Some animals such as molluscs and arthropods have blue blood because they utilize hemocyanin, a type-3 copper-containing protein that freely dissolves in hemolymph for oxygen transportation. Molluscan hemocyanins form decamers or multidecamers of 330–550 kDa subunits, which associate into huge cylindrical supermolecules with molecular masses varying from 3.5 to 13.5 MDa. Subunits of most molluscan hemocyanins consist of an N-terminal segment of six paralogous functional units (FUs; a-b-c-d-e-f) and a C-terminal segment with a varying number of FUs. Ten copies of the N-terminal segment (FUs a, b, c, d, e and f) thereby form a conserved cylinder wall, whereas the C-terminal segments form several inner-collar domains, located on the inner periphery of the cylinder.

Type 4 molluscan hemocyanin (squid type) is exceptional since this is the only molluscan hemocyanin type with an additional FU (FU-d*) within the N-terminal segment that usually forms the cylinder wall. Therefore, we constructed the entire structure model by rigid-body fitting. Our structure revealed a striking asymmetric inner-collar architecture and a conserved symmetric cylinder wall. 5 symmetry that is shifted towards one cylinder opening (northern hemisphere of the lumen). In TpH, the FU-gs form typical FU dimers, but in this case the dimers unusually occupy the northern and southern hemispheres of the inner space alternately [cyan FUs in Figs. 1(e) and 2(b)]. FU-d*s do not form dimers, instead single copies fill void spaces between the FU-g dimers. The segment of the wall FUs (a-b-c-d,e-f) is invariant for all ten protomers and there are two different possible conformations for each FU-g and FU-d* within a single protomer, thereby resulting in four different protomer types, namely conformers 1, 2, 3 and 4.

>[10x]NLLRKNVDTLTPDEILNLQVSLRAMQDDEGASGYQAISAYHGEPADCKAADGSTIVCCLHGMPTFPMWHRLYLVQFEQALVAHGSTLGIPYWDWTKPMTQLPELVQHPLFIDPTGKKAKKNVFYSGEIKFENKVTARAVDARLYQASQEGQKNFLLEGVLNALEQEDFCHFEVQLEVAHNPIHYLVGGRFTHSMSSLEYTSYDPLFFLHHSNVERHFALWQALQKHRGLPTRPNCGLNLFHSPMEPFGRDTNPFAITKDNSKASSLFDYEHLGYAFDDLSLNGMTIEELEALLKQRRSGARAFANFRLGGIKTSANVRIKLCIPTEDKRQSDNCDNDAGQFFILGGTNEMPWNFAFPYLHEITDTVLSLGLALDSNYYVTAEVTAINGTLMPTQTIPRPIVTYIPPQGFKDVNMVNMDTSSLRFRKDISSLTTEEEYELRVAMERFMSDKSINGYQALAEFHGLPAKCPRPDALNRVACCIHGMATFPHWHRLVVMQFENALFTRGSPIGVPYWDWTKPFTALPSLLADETYVDPYTKETKPNPFFKAPIEFLKAGVHTSRQIDERLFKQPSKGDHGFLYDGLSLAFEQDDFCDFEVQFEVTHNSIHAWTGGSEPYSMSSLHYTSFDPMFWLHHSQVDRLWAIWQALQIQRGKPYKTYCANSEVYRPMKPFAFKSPLNNDEKTREHSVPTDVYDYQAELAYTYDTLFFGGLSIRELQRYVEEAKSKDRVFAGFLLMGIQTSANVDLFVVAGGNEFFVGSIAVLGGSKEMTWRFDRVYKHEITDALGALGVDMFAEYTLRVDIKDVNGTALPPTAIPPPIVIFVPGIADANVKFDEQHRSRKNVDSMTVSEMNALRTAMAAFAADKEVTGYQQVAAFHGSTQWCPSPDAAQKYACCHHGMATFPHWHRLIALNFENGLRRNGWSGGLPYWDWTRPIDALPALVLEAEYTDANGEAKPNPFFSGAIDSIGASTSRAPTEALYEKPDFGKYTHLANEIISALEQEDFCDFEVQYEIAHNHIHALVGGTEAVSMASLEYSAFDPIFMLHHSNVDRIWATWQALQKFRGKAYNSANCAIEILRKPMSPFSLASDINPDAMTREYSVPFDVFNYKKNFHYEYDTLELNGLSIXQLSREINRRKAKNRVXVTFMLEGLKKSLLVEYFIAADGTDQKMKAGEFYVLGSENEMPWKFDRPYKSDITYVMDAMKLHYTDKYHVELRITDMTGAEVTDLKLVTSVIYEPGIGNFGEGRRWISPITSASRIRKNLLDFEDGEMESLRNAFKQMADEGRYEEIASFHGVPAQCPSEDGTMVHTCCLHGMPVFPHWHRLYVSLVEDELLARGSGVAVPYWDWVEPFDELPRLINEATFYNSRTLQIEPNPFFKGKISFENAETDRDTQPELFGNRYLYDHTLFVFEQTDFCEFEVHYEVLHNTIHSWLGGRDVHSMSSLDYAAYDPVFFLHHSNVDRLWAIWQELQRYRKLSYNEANCALPLMNQPMRPFSNSTANNDRLTFTNSRPNDVFDYQNVLHYKYDTLNFAGLSIPQLERILQKNQGRDRIFAGFLLHGIKASADVRIYICVPTGIGEENCGNYAGIFSVLGGETEMPWQFDRLFRYEITDELKKLGLNQNSHFRVEMELTAVNGSKITQKIFPNPTIIFVPSDVEFEEDTWRDVVTSANRIRRNLKDLSKEDMFSLRAAFKRMTDDGRYEEIAAFHGLPAQCPNADGSNIHTCCLHGMPTFPHWHRLYLSLVENELLARGSDVAVPYWDWIEPFDSLPGLISDETYKHPKTNEDIENPFHHGKISFADAVTVRKPRDQLFNNRYLYEHALFAFEHTDFCDFEVHFEVLHNSIHSWIGGPNPHSMSSLDFAAYDPIFFLHHSTVDRLWAIWQDLQRYRKLDYNVANCALNLLNDPMRPFNNKTANQDHLTFTNSRPNDVFDYQNSLNYKFDSLSFSGLSIPRLDDLLESRQSHDRVFAGFWLSGIKASADVNIHICVPIGVEHEDCDNYAGTFAVLGGETEMPWAFDRLFRYEISDEMKKLQLTEDSKFRLTTNIIASNGSKVSNDIFPTPTVIFVPKKERTEQVSTTKSVRGNLVRKNVDRLSLQEINSLIHALKRMQKDRSSDGFETIASFHALPPLCPNPTAKHRHACCLHGMATFPQWHRLYVVQFEHSLNRHGAIVGVPYWDWTYPMTEVPGLLTSEKYTDPFTGIETFNPFNHGHISFISPETMTTREVSEHLFEQPALGKQTWLFNNIILALEQTDYCDFEVQFEIVHNSIHSWLGGKELYSLNHLHYAAYDPAFFLHHSNVDRLWVVWQELQKFRGLPAYESNCAIELMSQPLKPFSFGAPYNLNPVTTKYSKPSDVFNYKQNFHYEYDMLEMNGMSIAQLESYIRQERQKDRVFAGFLLEGFGSSAYATFQVCPDVGDCYEGSHFSVLGGSTEMPWAFDRLYKMEITDILQAMDLKFDSHFTIKTKIVAHNGTELPESLLPEATIVRIPPSAQNLEVAIPLNRIRRNINSLESRDVQNLMSALKRLKEDESDFGFQTIAGYHGSLMCPTPEAPEYACCLHGMPTFMHWHRVYLLHFEESMRRHGASVAVPYWDWTMPSDNLPSLLGDADYYDAWTDSVIENPFLRGHIKYEDTYTVREIQPELFALAEGQKESTLFKDVMLMFEQEDYCDFEVQAEVIHNSIHYLIGGHQKYAMSSLMFSSFDPIFYVHHSMVDRLWAIWQELQKHRKLPHDKAYCALDQMAFPMKPFIWESNPNPTTRAVSTPSKLFDYKSLGYDYDHLNFHGMSIGQLEALIQKQKKADRVFAGFLLHGIKISADVHLKICIEADCQEAGVIFVLGGETEMPWHFDRNYKMDITDVLKKRNIPPEALFEHDSKIRLEVEIKSVDGAVLDPNSLPKPSLIYAPAKGLIIQQVGEYDAGSMVRKNVNSLTPSEIENLRNALAAVQADKTDAGYQKIASFHGMPLSCQYPDGTAFACCQHGMVTFPHWHRLYMKQMEDALKAKGAKIGIPYWDWTTAFHSLPILVTEPKNNPFHHGYIDVADTKTTRDPRPQLFDDPEQGDQSFFYRQIAFALEQRDFCDFEIQFEMGHNAIHSWVGGPSPYGMSTLHYTSYDPLFYVHHSNTDRIWAIWQALQKYRGLPYNSANCEINKLKKPMMPFSSEDNPNEVTKAHSTGYKSFDYQQLNYEYDNLNFHGMTIPQLEVHLKKIQEKDRVFAGFLLRAIGQSADVNFDVCRKDGECTFGGTFCVLGGDYEMPWAFDRLFLYDISKSLVHLRLDAHDDFDIKVTIMGIDGKSLPPNLLPSPTILFKPGTGKI>MQTPHILIVEDELVTRNTLKSIFEAEGYDVFEATDGAEMHQILSEYDINLVIMDINLPGKNGLLL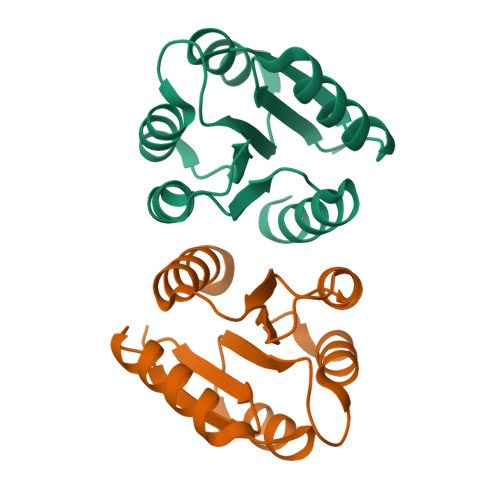ARELREQANVALMFLTGRDNEVDKILGLEIGADDYITKPFNPRELTIRARNLLSRTMQ[2x]> STAAGQERREKLTEETDDLLD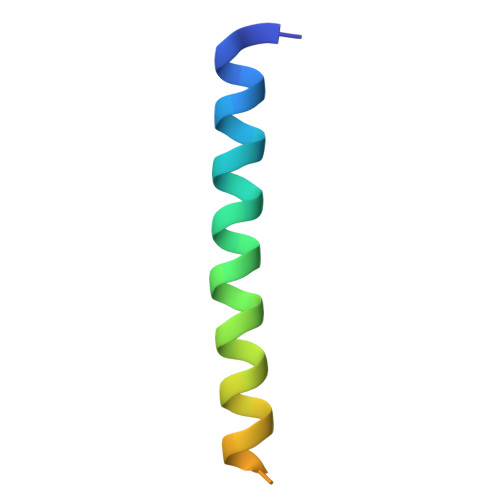EIDDVLEENAEDFVRAYVQKGGE Olfactomedin-1 (Olfm1; also known as Noelin or Pancortin) is a highly-expressed secreted brain and retina protein and its four isoforms have different roles in nervous system development and function. Structural studies showed that the long Olfm1 isoform BMZ forms a disulfide-linked tetramer with a V-shaped architecture. The tips of the Olfm1 “V” each consist of two C-terminal β-propeller domains that enclose a calcium binding site. The highly conserved monomeric Olf domain has a five-bladed β-propeller fold with a central metal ion binding site.

Based on our previous structure, we designed truncations that are expected to result in a monomeric domain by truncating the dimerizing coiled coil and excluding Cys221 from the construct (the Olfm1Olf construct includes UNIPROT residues 226–478). We determined a high-resolution crystal structure of Endo-H-deglycosylated Olfm1Olf, which leaves a single acetylglucosamine (GlcNAc) attached to glycosylated asparagines. Our best crystal diffracted to 1.25 Å resolution, representing the highest resolution crystal structure of an Olfactomedin domain to date. Because of the high resolution of our Olfm1Olf diffraction data to 1.25 Å, we can unambiguously assign a Na+ and a Ca2+ ion bound in the central cavity of the β-propeller. Metal ion assignment was based on previous binding data, coordination distances and fit to the electron density. The Ca2+ ion is coordinated by the negatively-charged carboxyl groups of the side chains of Asp356, Asp453 and Glu404, as well as by the backbone carbonyl groups of Ala405 and Leu452 and a single water molecule (Fig. 4b and Table 2 for coordination distances and angles). The Na+ ion is also coordinated by the carboxylic acid groups of the side chains of both Asp356 and Asp453, as well as by the backbone carbonyl group of Leu357 and a different water molecule than the one coordinating the calcium ion. The conserved residue Tyr347 stabilises the switch loop by forming a hydrogen bond between the Tyr347 hydroxyl group and the Asp356 carboxyl group (distance 2.7 Å) that plays a central role in coordinating both the bound sodium and calcium ions. The high-resolution crystal structure of Olfm1Olf reveals a hydrophilic tunnel filled with water molecules running from the surface of the Olf domain to the metal ion binding sites. In Olfm1, the tunnel starts at the solvent-exposed top face between propeller blade 2 and 3 and runs between these two blades towards the metal ion binding sites. Twelve ordered water molecules are well resolved in this tunnel due to the high resolution of our electron density map, including the two water molecules involved in coordinating the Na+ and Ca2+ ions.

> GSACGKLTGISDPVTVKTSGSRFGSWMTDPLAPEGDNRVWYMDGYHNNRFVREYKSMVDFMNTDNFTSHRLPHPWSGTGQVVYNGSIYFNKFQSHIIIRFDLKTETILKTRSLDYAGYNNMYHYAWGGHSDIDLMVDENGLWAVYATNQNAGNIVISKLDPVSLQILQTWNTSYPKRSAGEAFIICGTLYVTNGYSGGTKVHYAYQTNASTYEYIDIPFQNKYSHISMLDYNPKDRALYAWNNGHQTLYNVTLFHAAAHHHHHH>HGEKSQQAFLRMRTLNWYDVKWSKTSLNVNESMVLSGKVHVFSAWPQAVANPKSSFLNAGEPGPVLVRTAQFIGEQFAPRSVSLEVGKDYAFSIDLKARRAGRWHVHAQINVEGGGPIIGPGQWIEIKGDMADFKDPVTLLDGTTVDLETYGIDRIYAWHFPWMIAAAAWILYWFFKKGIIASYLRISEGKDEEQIGDDDRRVGAIVLAVTILATIIGYAVTNSTFPRTIPLQAGLQKPLTPIIEEGTAGVGPHVVTAELKGGVYKVPGRELTIQVKVTNKTDEPLKLGEYTAAGLRFLNPDVFTTKPEFPDYLLADRGLSTDPTPLAPGETKTIEVKVQDARWDIERLSDLAYDTDSQIGGLLMFFSPSGKRYATEIGGPVIPKFVAGDMP[3x];>[3x]MFTSKSGGAIGPFHSVAEAAGCVKTTDWMFLTLLFLAVLGGYHIHFMLTAGDWDFWVDWKDRRMWPTVVPILGVTFAAAAQAFFWENFKLPFGATFAVSGLLIGEWINRYCNFWGWTYFPISLVFPSALVVPALWLDIIMLLSGSYVITAVVGSLGWGLLFYPNNWPAIAALHQATEQHGQLMSLADLVGFHFVRTSMPEYIRMVERGTLRTFGKEVVPVAAFFSGFVSMMVYFLWWFVGKWYSTTKVIQKI;>[3x]MSVTTETTAGAAAGSDAIVDLRGMWVGVAGLNIFYLIVRIYEQIYGWRAGLDSFAPEFQTYWLSILWTEIPLELVSGLALAGWLWKTRDRNVDAVAPREELRRHVVLVEW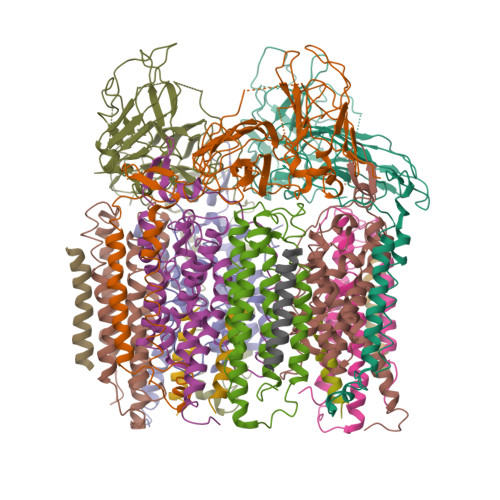LVVYAVAIYWGASFFTEQDGTWHMTVIRDTDFTPSHIIEFYMSYPIYSIMAVGAFFYAKTRIPYFAHGFSLAFLIVAIGPFMIIPNVGLNEWGHTFWFMEELFVAPLHWGFVFFGWMALGVFGVVLQILMGVKRLIGKDCVAALVG>MGRDPNSTNDTTTQNVVLTKYGFDKDVTAIDRATDQIWTGDGAKPLQGVDFTIYNVTANYWASPKDYKGSFDSAPVAATGTTNDKGQLTQALPIQSKDASGKTRAAVYLFHATNPRAGYNTSADFWLTLPAKAAADGNVYVYPKNVQKTTYERTFVKKDAETKEVLEGAGFKISNSDGKFLKLTDKDGQSVSIGEGFIDVLANNYRLTWVAESDATVFTSDKSGKFGLNGFADNTTTYTAVETNVPDGYDAAANTDFKADNSSSDILDAPSGILPLEHHHHHH[3x]

As the first reported host of “non-pathogenic-derived” pili, Lactobacillus rhamnosus GG is a gut-adapted commensal lactic acid bacterium (LAB) and one of many clinically investigated probiotic strains for human use in the prevention and treatment of certain gastric ailments. As with other Gram-positive bacteria, sortase-dependent piliation in L. rhamnosus GG (called SpaCBA) is assembled from the ~30 kDa SpaA (backbone), ~20 kDa SpaB (basal), and ~90 kDa SpaC (tip-located) pilins. Two immunoglobulin (Ig)-like subdomains comprise GG-SpaA, each having the conserved residues of a canonical E-box motif and internal isopeptide bonds formed between either lysine and asparagine or lysine and aspartate residues. Our findings show that the GG-SpaA structure has certain features in common with other pathogen-derived pilin-proteins, such as the Ig-like CnaB-type folds and the presence of internal isopeptide bonds6940.

The overall structure of the E139A-substituted mutant was quite similar to that of the WT GG-SpaA protein (RMSD of 2 Å). Discontinuous electron density was observed between Lys47 and Asn172 that can be attributed to the loss of the N-terminal isopeptide bond. The alanine substitution at residue position 139 was also apparent in the electron density map. Despite the overall fold of the E139A mutant being retained, some minor conformational variations are present near the mutation site, including the flexible AB loop region at the N-domain. For instance, individual side chains for the Asn172, Lys47, and Ser149 residues were now oriented differently due to the absence of the isopeptide bond and the subsequently altered hydrogen-bonding network. Here, the Asn172 side chain is repositioned closer toward the C-domain and thus able to form a hydrogen bond with the OH group of the Lys47 side chain. Moreover, the Ser149 side chain is rotated towards the domain interface. A water molecule, which is found in the place of the Glu139 side chain, is hydrogen bonded to the NH group of the Asn172 side chain. In addition, the slight shifting of the AB loop backbone has occurred, but with a major structural deviation (3 Å) at Gly69. Because the K-D isopeptide bond was held intact, the structure of the C-domain was seen to be largely unaffected.>[8x]MSSSEDKITVH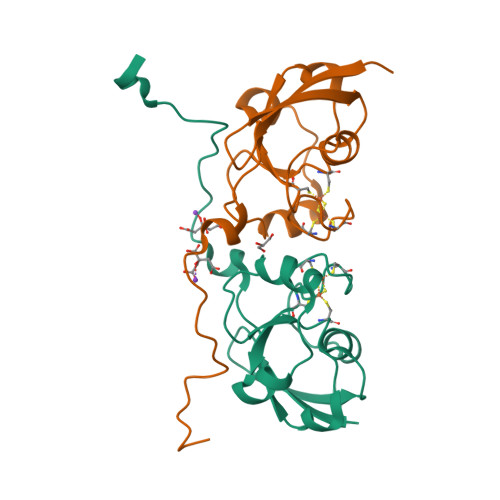FINRDGETLTTKGKVGDSLLDVVVENNLDIDGFGACEGTLACSTCHLIFEDHIYEKLDAITDEENDMLDLAYGLTDRSRLGCQICLTKSMDNMTVRVPETVADARQSIDVGKTSAENLYFQ>[3x]LHQLSSPRYKFNFIADVVEKIAPAVVHIELFLRHPLFGRNVPLSSGSGFIMSEAGLIITNAHVVSSNSAAPGRQQLKVQLQNGDSYEATIKDIDKKSDIATIKIHPKKKLPVLLLGHSADLRPGEFVVAIGSPFALQNTVTTGIVSTAQREGRELGLRDSDMDYIQTDAIINYGNAGGPLVNLDGEVIGINTLKVTAGISFAIPSDRITRFLTEFQDKQIKDWKKRFIGIRMRTITPSLVDE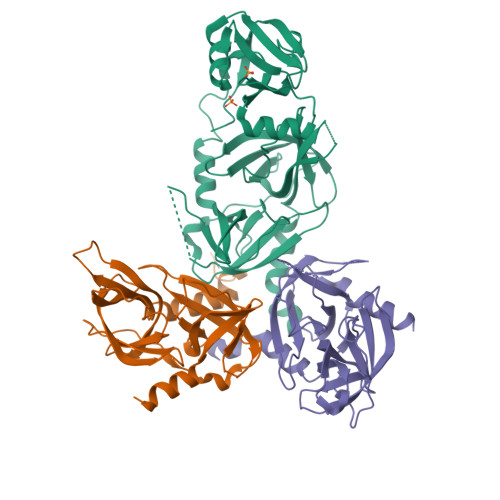LKASNPDFPEVSSGIYVQEVAPNSPSQRGGIQDGDIIVKVNGRPLVDSSELQEAVLTESPLLLEVRRGNDDLLFSIAPEVVMGGHHHHHH>[7x]ILPSFIEHSSFGVKESNPYNKLFEERIIFLGVQVDDASANDIMAQLLVLESLDPDRDITMYINSPGGGFTSLMAIYDTMQYVRADIQTVCLGQAASAAAVLLAAGTPGKRMALPNARVLIHQPSLSGVIQGQFSDLEIQAAEIERMRTLMETTLARHTGKDAG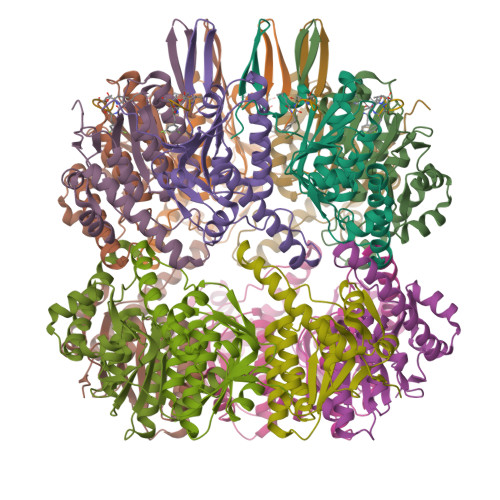VIRKDTDRDKILTAEEAKDYGIIDTVLEYRKLSAQTA;>[7x]MRSNSQGLSLTDSVYERLLSERIIFLGSEVNDEIANRLCAQILLLAAEDASKDISLYINSPGGSISAGMAIYDTMVLAPCDIATYAMGMAASMGEFLLAAGTKGKRYALPHARILMHQPLGGVTGSAADIAIQAEQFAVIKKEMFRLNAEFTGQPIERIEADSDRDRWFTAAEALEYGFVDHIITRAHVNGEAQ> GGGSVTKKRKLESTESRSSFSQHARTSGRVAVEEVDEEGKFVRLRNKSNEDQSMGNWQIKRQNGDDPLLTYRFPPKFTLKAGQVVTI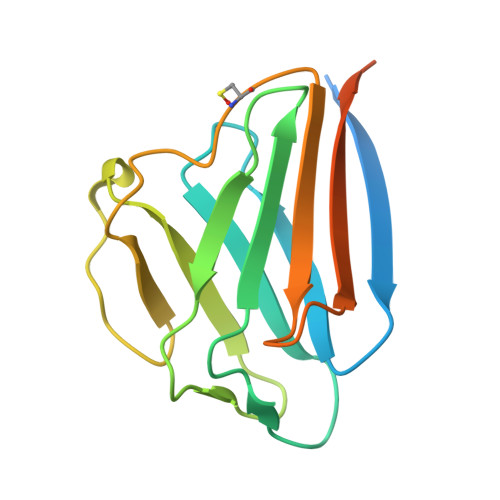WAAGAGATHSPPTDLVWKAQNTWGCGNSLRTALINSTGEEVAMRKLVRSVTVVEDDEDEDGDDLLHHHH>SNAMIIRPEQHWFLRLFDWHGSVLSKI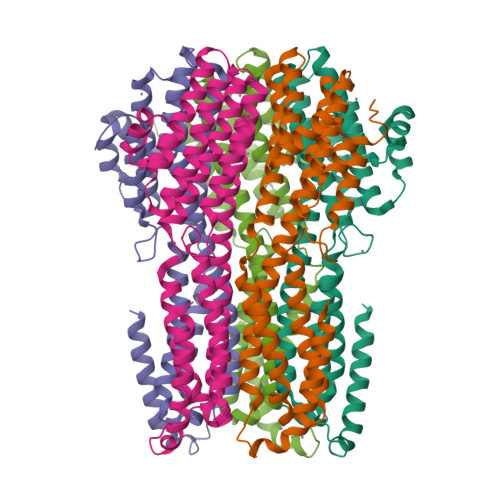IFRLLLNVLMSIIAIISYQWYEQLGIHLTVAPFSLLGIAIAIFLGFRNSASYSRFVEARNLWGTVLIAERTLVRQLRNILPAEHDAHRRIVSYLVAFSWSLKHQLRKTDPTADLRRLLPEERVTEILASSMPTNRILLLAGNEIGQLREAGKLSDITYGLMDNKLDELAHVLGGCERLATTPVPFAYTLILQRTVYLFCTLLPFALVGDLHYMTPFVSVFISYTFLSWDSLAEELEDPFGTAANDLPLNAMCNTIERNLLDMTGQHPLPETLRP[5x]>[6x]RGHHHHHHGSFTPSGTTGTTKLTVTEKCQVRVGDLTVAKTRGQLTDA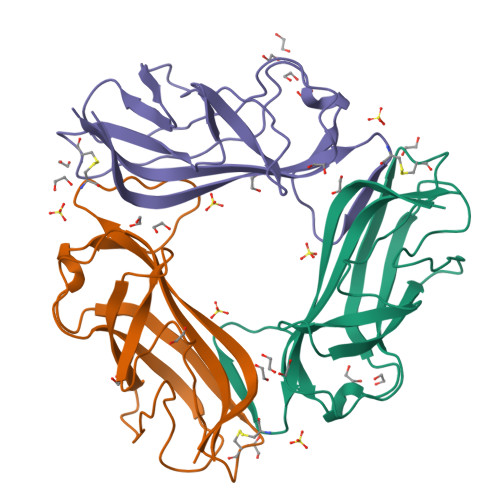APIGPVTVQALGCDARQVALKADTDNFEQGKFFLISDNNRDKLYVNIRPTDNSAWTTDNGVFYKNDVGSWGGIIGIYVDGQQTNTPPGNYTLTLTGGYWAK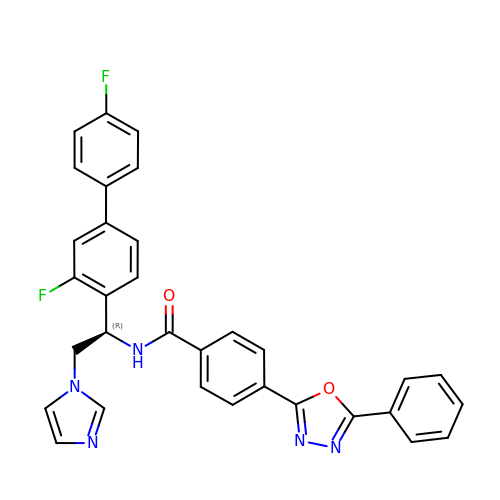N-[(1R)-1-(3,4'-difluorobiphenyl-4-yl)-2-(1H-imidazol-1-yl)ethyl]-4-(5-phenyl-1,3,4-oxadiazol-2-yl)benzamide | C32 H23 F2 N5 O2 | YTJXXDVLDUKYHV-LJAQVGFWSA-N Signaling by the human C-type lectin-like receptor, natural killer (NK) cell inhibitory receptor NKR-P1, has a critical role in many immune-related diseases and cancer. Human NKR-P1 and LLT1 are type II transmembrane glycoproteins with similar protein topology: an N-terminal cytoplasmic signaling tail, a transmembrane helix, a flexible stalk region, and a C-terminal C-type lectin-like domain (CTLD). In addition, NKR-P1 promotes transendothelial migration to immunologically privileged niches upon interaction with its endogenous ligand, lectin-like transcript 1 (LLT1). Here we report the crystal structures of the NKR-P1 and NKR-P1:LLT1 complexes, which provides evidence that NKR-P1 forms homodimers in an unexpected arrangement to enable LLT1 binding in two modes, bridging two LLT1 molecules.

The asymmetric unit of NKR-P1_glyco contains two monomers, whereas the asymmetric unit of NKR-P1_deglyco contains eight NKR-P1 monomers. All these monomers are arranged into very similar homodimers, with pairwise RMSD on Cα atoms up to 0.5 Å. Glycosylation at Asn169 is visible in the electron density maps of both NKR-P1_glyco and _deglyco structures. In NKR-P1_glyco, the complete GlcNAc2Man5 carbohydrate chain is localized in chain A, whereas a partial GlcNAc2Man3 chain is localized in chain B. Interestingly, the localized first GlcNAc units linked at Asn116 in NKR-P1_glyco and the overlapping GlcNAc units at Asn116 and Asn157 remaining in NKR-P1_deglyco participate in dimerization contacts with residues of helices α1 and regions β2, L1, and β2’ of the opposite subunit of the NKR-P1 homodimer. In NKR-P1_glyco, five hydrogen bonds between Asn116:GlcNAc and the opposite subunit stabilize the helix α1-centered homodimer. The contact surface area between the opposite chain of NKR-P1 and the localized GlcNAc unit is approximately 125 Å2. Conversely, in NKR-P1_glyco, the first GlcNAc unit at Asn116 is well defined in electron density in both chains, A and B, of the NKR-P1 dimer, while no electron density was found for glycosylation at Asn157. This suggests that although the glycosylation on either Asn116 or Asn157 can contribute to the dimer formation, dimerization might be impaired by steric hindrance if both N-glycans are present simultaneously.

>[2x]ETGGLLNCPIYWQQLREKCLLFSHTVNPWNNSLADCSTKESSLLLIRDKDELIHTQNLIRDKAILFWIGLNFSLSEKNWKWINGSFLNSNDLEIRGDAKENSCISISQTSVYSEYCSTEIRWICQKELTPVRNKVYPDSKHHHHHH(6S)-1-(2,3-dihydro-1,4-benzodioxin-6-yl)-6-{(5M)-5-(3,5-dimethyl-1,2-oxazol-4-yl)-1-[(1s,4R)-4-methoxycyclohexyl]-1H-benzimidazol-2-yl}piperidin-2-one | C32 H36 N4 O5 | 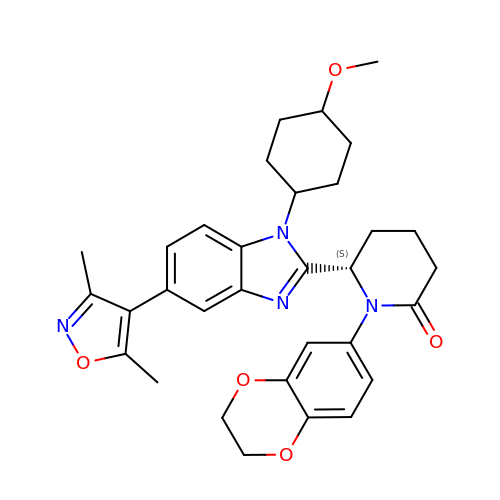ZVVSHSLAQZHUJM-LLGBQNBKSA-N>MPTLLRVYIDGPHGMGKTTTTQLLVALGSRDDIVYVPEPMTYWRVLGASETIANIFTTQHRLDQGEISAGDAAVVMTSAQITMGMPYAVTDAVLAPHIGGEAGSSHAPPPALTLIFDRHPIAALLCYPAARYLMGSMTPQAVLAFVALIPPTLPGTNIVLGALPEDRHIDRLAKRQRPGERLDLAMLAAIRRVYGLLANTVRYLQCGGSWREDWGQLSGTAVPPQGAEPQSNAGPRPHIGDTLFTLFRAPELLAPNGDLYNVFAWALDVLAKRLRSMHVFILDYDQSPAGCRDALLQLTSGMVQT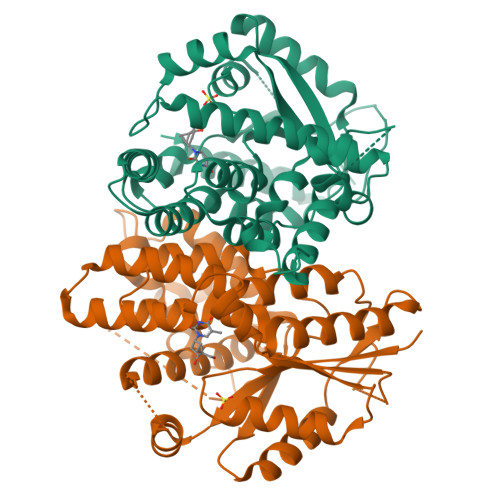HVTTPGSIPTICDLARTFAREMGEAN[2x]2',5'-dideoxyadenosine 3'-(tetrahydrogen triphosphate) | C10 H16 N5 O11 P3 | 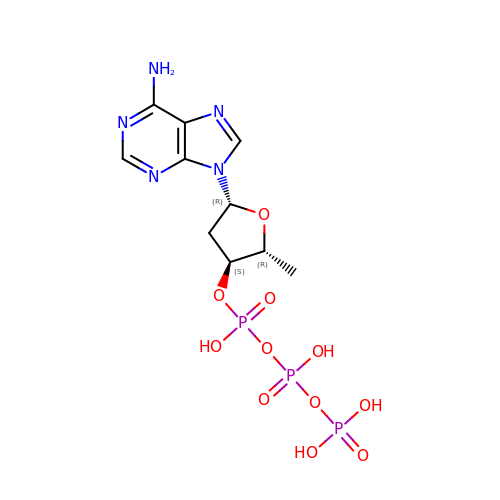ZJGUOEYCABTFNH-DSYKOEDSSA-N> MSQFTLYKNKDKSSAKTYPYFVDVQSDLLDNLNTR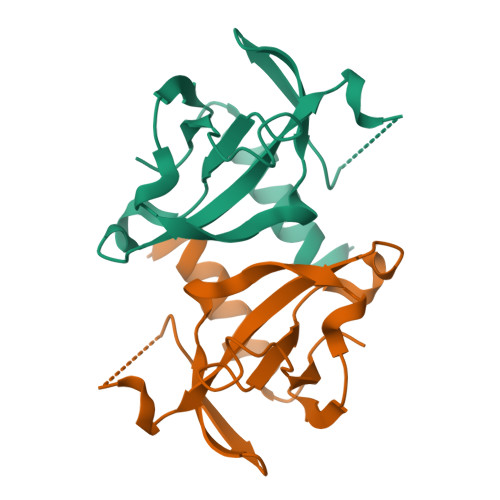LVIPLTPIELLDKKAPSHLCPTIHIDEGDFIMLTQQMTSVPVKILSEPVNELSTFRNEIIAAIDFLITGI(3R,5R)-5-{3-[4-(trifluoromethyl)phenyl]-1,2,4-oxadiazol-5-yl}pyrrolidin-3-ol | C13 H12 F3 N3 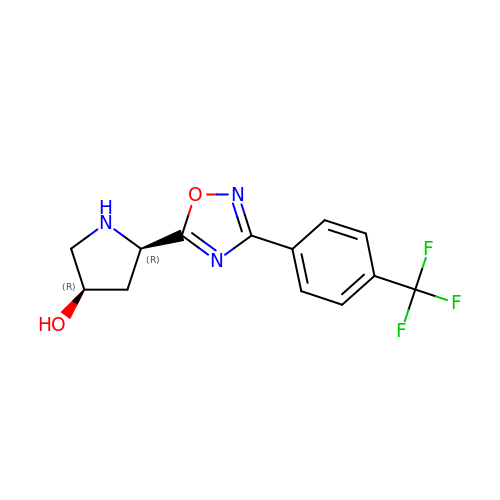O2 | BFYYUFJLDXZELT-NXEZZACHSA-N In the present work, we focus on a class of monocyclic disulfide‐containing 19 amino acid peptides targeting the Vascular Endothelial Growth Factor‐A, the main pro‐angiogenic factor in Human. We proposed to use this peptide as a model to rationalize the thermodynamics of α‐helix stabilization by an i to i+4 lactam bridge. Around 950 Å2 of accessible surface area (ASA) was buried at the peptide‐VEGF interface, that overlapped with the VEGF receptor 1 domain 2 (VEGFR1‐d2)‐binding site. Although only lactam‐bridged ExxxK, DxxxK and KxxxD induced the formation of stable helix in the unbound state, all peptides of the series were helically folded when bound to VEGF.

Constraints caused by the lactam bridges and by the binding of the macro‐cyclized peptide to the VEGF site also made the α‐helices non‐canonical: in each of the four peptides, the residues P8‐11 folded into a 310‐helix characterized by a H‐bond between Glu P8 O and Cys P11 HN. For the peptides 1 c and 2 c (KxxxD and DxxxK), the DSSP software identified residues P9‐14 as an α‐helix, although Trp P9 O could bind to both Phe P12 HN and Glu P13 HN. No steric conflict was observed on peptide 2 c. However, the NMR structure calculations did not converge into a single conformation. The backbone RMSD of the 20 lowest energy NMR structures, compared to the co‐crystal structures of bicyclic peptides and VEGF (see below), indicated that the bicyclic 2 c and 3 c were significantly closer to the folded structures than were the other peptides. Helical folds were observed in most structures for 2 c and 3 c, resulting in a single α‐helical cluster for a RMSD cutoff of 1.2 Å. The overall analysis by spectroscopic methods also evidenced that 2 c was the most structured peptide in solution with 3 c. However, in our data, the stabilization of α‐helix by the lactam bridge directly improved the affinity but did not correlate with an entropy gain: the affinity of 4 c was slightly decreased despite an entropy gain, and the binding of peptide 2 c to VEGF exhibited a less favorable entropy variation than peptide 2, despite the high helicity of unbound peptide 2 c and improved affinity. An explanation could be a difference in ΔS°solv between peptides 2 c and 2, but the ΔCp of both peptides did not evidence any significant variation in the desolvation process upon binding to VEGF. Moreover, the apparent inconsistency of entropy changes in peptides 2/2 c likely results from differences in vibrational entropy due to the cyclization constraints. We propose that the vibrational entropy decreases when the flexibility of the conformation of the bound bicyclic peptide decreases, i. e. when the free energy well is narrowed.

> CDIHVLWEWDCFEKLX;>[2x]EVVKFMDVYQRSYCHPIETLVDIFQEYPDEIEYIFKPSCVPLMRCGGCCNDEGLECVPTEESNITMQIMRIKPHQGQHIGEMSFLQHNKCECRPK>AHNNENVSGISAYLLGLIIGDGGLYKLKYKGNRSEYRVVITAKSENLIKQHIAPLMQFLIDELNVKSKIQIVKGDTRYELRVSSKKLYYYFANMLERIRLFNMREQIAFIKGLYVAEGDMTLKRLRIWNKNKALLEIVSRWLNNLGVRNTIHLDDHRHGVYVLNISLRDRIKFVHTILSSHLNPLPPEAAALEHHHHHH[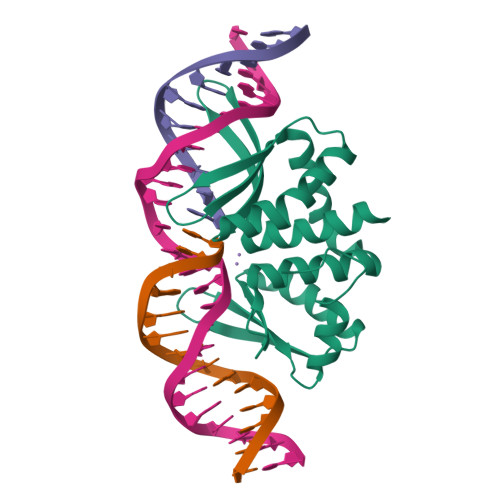3x]>MHHHHHHMFSRFSNVVSEIEKKYVDKISISEIMTKAIEGLLSNLDAHSAYLNEKKFKEFQAQTEGERGGLGITVGMRDGVLTVIAPLEGTPAYKAGVKSGDNILKINNESTLSMSIDDAINLMRGKPKTPIQITIVRKNEPKPLVFNIIRDIIKLPSVYVKKIKETPYLYVRVSGFDKNVTKSVLEGLKANPKAKGIVLDLRGNPGGLLNQAVGLSNLFIKEGVLVSQKGKNKEESLEYKANGRAPYTNLPIAVLVNGGSASASEIVAGALQDHKRAVIIGEKTFGKGSVQMLLPVNKDEAIKITTARYYLPSGRTIQAKGITPDIVIYPGKVPEN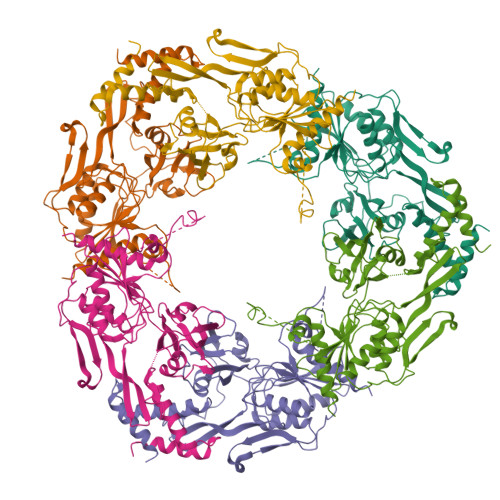ENKFSLKEADLKHHLEQELKKLDDKTPNSKEADKDKKNEEEKEVTPKMINDDIQLKTAIDSLKTWSIVDEKMDEKAPKKK[4x]2-Aminopurine riboside-3',5'-cyclic monophosphate | C10 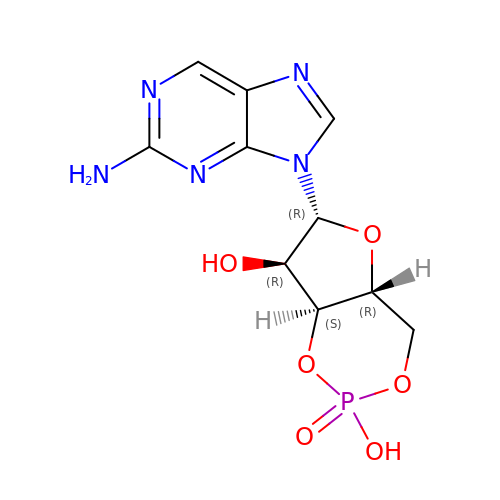H12 N5 O6 P | ZZUVWWINFTZMGV-JXOAFFINSA-N>[4x]LTQELGTAFFQQQQLPAAMADTFLEHLCLLDIDSEPVAARSTSIIATIGPASRSVERLKEMIKAGMNIARLNFSHGSHEYHAESI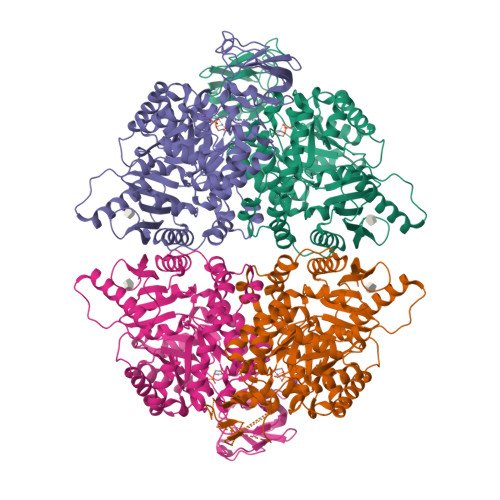ANVREAVESFAGSPLSYRPVAIALDTKGPEIRTGILQGGPESEVELVKGSQVLVTVDPAFRTRGNANTVWVDYPNIVRVVPVGGRIYIDDGLISLVVQKIGPEGLVTQVENGGVLGSRKGVNLPGAQVDLPGLSEQDVRDLRFGVEHGVDIVFASFVRKASDVAAVRAALGPEGHGIKIISKIENHEGVKRFDEILEVSDGIMVARGDLGIEIPAEKVFLAQKMMIGRCNLAGKPVVCATQMLESMITKPRPTRAETSDVANAVLDGADCIMLSGETAKGNFPVEAVKMQHAIAREAEAAVYHRQLFEELRRAAPLSRDPTEVTAIGAVEAAFKCCAAAIIVLTTTGRSAQLLSWYRPRAAVIAVTRSAQAARQVHLCRGVFPLLYREPPEAIWADDVDRRVQFGIESGKLRGFLRVGDLVIVVTGWRPGSGYTNIMRVLSIS> MGSSHHHHHHSQDMEAAIEFDEIVKKLLNIYINDICTTGEKRLLNNYEKSILDRIYKSCEYIKKNYELDFNSMYNQININNITTSDIKSKIIEALLIDSRPSVKLATLSFISLIAEKWGEKNRAKIMEILSNEIVEKISNNGKDFIDFIDRDDDDIVDDYVL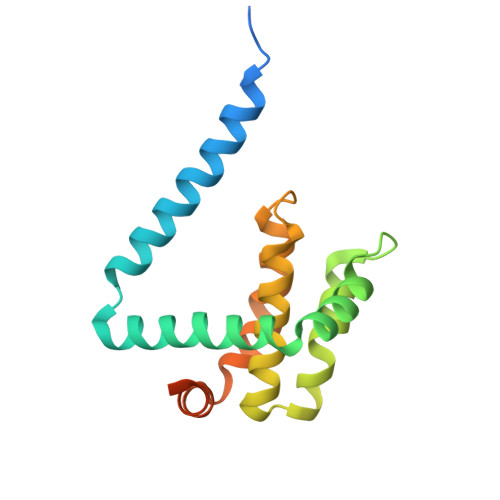ITNYLK> NEQSGISQTV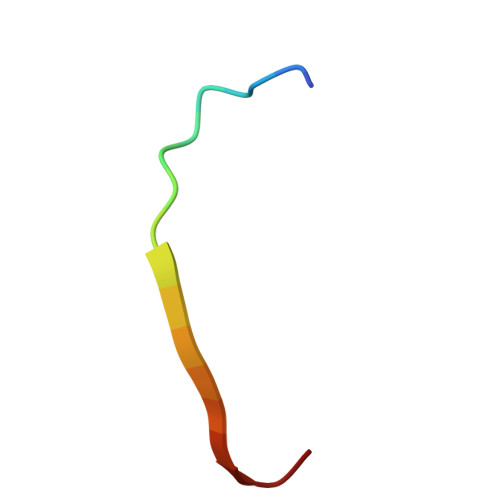IVGPWGAK>SSVASALLLQEAQAGFCRVDGTIDNNHTGFTGSGFANTNNAQGAAVVWAIDATSSGRRTLTIRYANGGTANRNGSLVINGGSNGNYTVSLPTTGAWTTWQTATIDVDLVQGNNIVQLSATTAEGLPNIDSLSVVGGTVR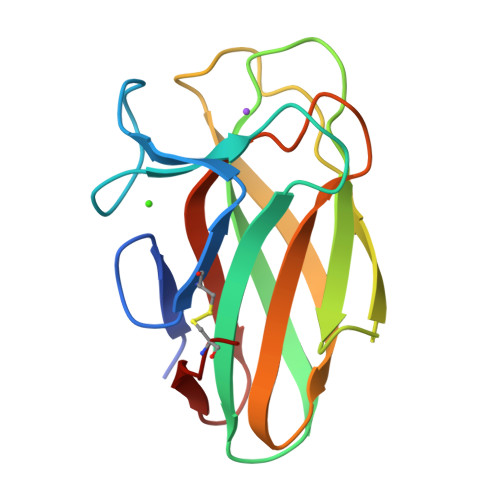AGNCG[2x]Gene transfer agents (GTAs) are DNA-containing phage-like particles produced by some species of bacteria and archaea. The genes encoding proteins that form Rhodobacter capsulatus GTA particles (RcGTA) are derived from phage DNA, which has been integrated into the bacterial genome. Here, we use cryo-electron microscopy (cryo-EM) to determine the structures of RcGTA before and after DNA ejection, and to visualize the interactions of RcGTA with R. capsulatus cells. Particles of RcGTA have heads with a diameter of 38-nm and 49-nm long tails.

The structures of the stopper, tail terminator and tail tube proteins have been determined to a resolution of 3.6 Å, and that of the distal tail protein to 4.0 Å. The attachment of distal tail proteins to tail tube proteins is enabled by the long loop of the tail tube protein, which interacts with the β2-core α-helix loop and short loop of the distal tail protein. The long loop of the tail tube protein mediates interactions between the tail tube proteins from successive discs and between the tail tube protein and distal tail protein. The insertion domain of the distal tail protein was resolved to a resolution of 5 Å and can adopt several conformations, as seen in two-dimensional class averages of RcGTA tails. The insertion domain of this RcGTA protein is homologous to that from the distal tail protein of phage T5, which has an oligosaccharide-binding fold. Therefore, it is possible that the insertion domain enables the binding of RcGTA particles to a sugar receptor at the cell surface of R. capsulatus, and flexibility of the domain may facilitate binding. Attachment of the RcGTA baseplate to the tail is enabled by the binding of the attachment domain of the hub protein and central domain of the megatron protein to the N-terminal Ala2, long loops, and C-terminal Arg209 of the distal tail proteins. The mismatch between the six-fold symmetry of the tail and threefold symmetry of the baseplate is resolved by the different conformations of residues from the long loops of odd and even subunits of distal tail proteins, which enable them to interact with hub and megatron proteins, respectively.

>MAAQNGKDLLIKLDLTGSGQFETIAGLRATRISFNAETVDVTSLESQGGWRELLGGAGVRSASISGAGVFKDADTDERARQIFFDGEVPEFQVIIPDFGIVQGPFMITSIDYAGSHNGEASYELAMASAGALSFTAI[2x];>MAFHEVRFPANLSFGSVGGPERRTEIVTLSSGHEERNSPWAHSRRHYDAGVGLRSLDDVERLIAFFEARGGQLHGFRWKDWADFKSCPASRAVAHEDQLIGMGDGVTTAFQLVKTYVSGGQSYLRPIVKPVEGTVKLGIAGDHQAEAVNFAVDHATGIVSFNEPPPQGARVTAGFEFDVPVRFDTDRIAVSVQSFQAGDLPQVPVVEVRI[2x]>IVPTRELENVFLGRCKDYEITRYLDILPRVRSDCSALWKDFFKAFSFKNPCDLDLGSYKDFFTSAQQQLPKNKVMFWSGVYDEAHDYANTGRKYITLEDTLPGYMLNSLVWCGQRANPGFNEKVCPDFKTCPVQARESFWGMASSSYAHSAEGEVTYMVDGSNPKVPAYRPDSFFGKYELPNLTNKVTRVKVIVLHRLGEKII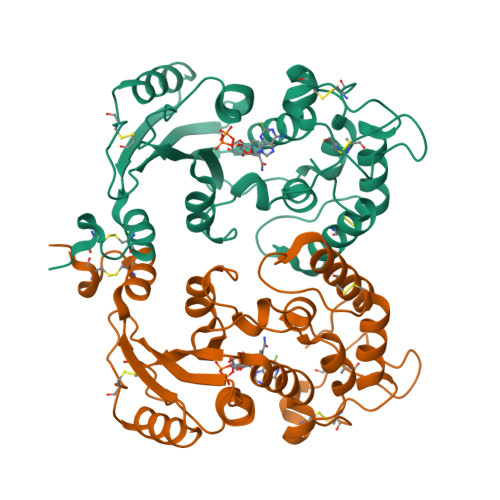EKCGAGSLLDLEKLVKAKHFAFDCVENPRAVLFLLCSDNPNARECRLAKRFYRIA[2x]> MRNKIFISHATPDDNDFTRWLALKLIGLGYEVWCDILFLDKGVDFWSNIEKVIREDTCKFLLVSSSYSNQREGVLKELAVAAKVKKQLKDDKFIIPLAIDEQLSYDDINIDIVRLNAIDFKMSWARGLKDILEAFEKQKVPKEVADASKSNLLYQQIFLHDKSVIEKEEIYDSNWLSILSFPEELRFHEYNWMLPKRFDVRELTFPAVRYKNYLCTFAWAYDFTYHLPKTETYHKSKTIRIPTEEILSGSYDSNFIRNAECKRLIVQLLNKAFELRMKDKEVQEYEMSNKTAYWLEKGKLEKDKFEKTMLVGKQKDKNWHFAISGASKLYPFPVLMISSHIFFTADGKKLIDSSSVQHSSRRRQGKNWWNNTWRTKL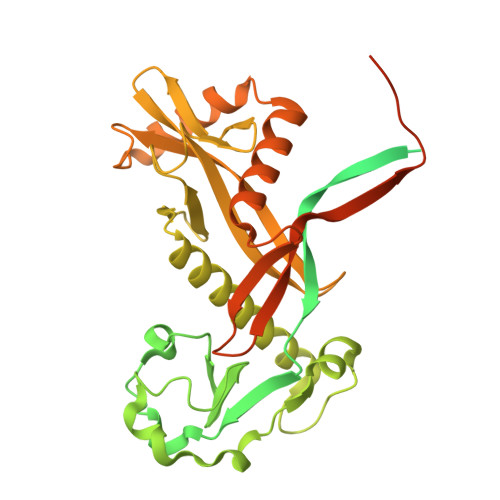LAFIKYLSDDDTSFYLEMGSEEKVFVSNEPVKFKGNVSYNIPEKNTLEEEAELSGFNQGEDIEELEELIENLEAE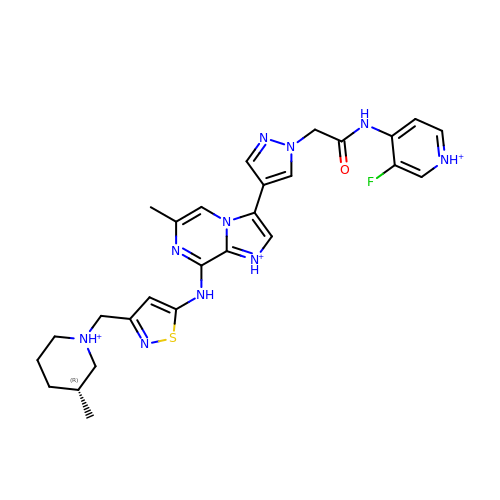3-(1-{2-[(3-fluoropyridinium-4-yl)amino]-2-oxoethyl}-1H-pyrazol-4-yl)-6-methyl-8-[(3-{[(1R,3R)-3-methylpiperidinium-1-yl]methyl}-1,2-thiazol-5-yl)amino]imidazo[1,2-a]pyrazin-1-ium | C27 H32 F N10 O S | PBHYAPKEUOBQSL-QGZVFWFLSA-Q>MERPQPDSMPQDLSEALKEATKEVHTQAENAEFMRNFQKGQVTRDGFKLVMASLYHIYVALEEEIERNKESPVFAPVYFPEELHRKAALEQDLAFWYGPRWQEVIPYTPAMQRYVKRLHEVGRTEPELLVAHAYTRYLGDLSGGQVLKKIAQKALDLPSSGEGLAFFTFPNIASATKFKQLYRSRMNSLEMTPAVRQRVIEEAKTAFLLNIQLFEELQELLTHDTKDQSPSRA[2x]

The heme oxygenase (HO) system comprises two active isozymes (HO-1 and HO-2) which are involved in the regioselective, oxidative cleavage of heme at the α-meso carbon. Cleavage results in the release of equimolar amounts of the gasotransmitter carbon monoxide (CO), ferrous iron (Fe2+), and biliverdin, the latter of which is reduced further by biliverdin reductase to form bilirubin. Of the two active isozymes, HO-1 is a ∼32 kDa stress protein found to be predominantly expressed in the spleen and inducible by a variety of stimuli including heat shock, heavy metals, heme and reactive oxygen species (ROS). Our laboratory has been focused on a program aimed at the design of novel, non-porphyrin based, isozyme-selective HO inhibitors based on the structure of (2S, 4S)-2-[2-(4-chlorophenyl)ethyl]-2-[(1H-imidazol-1-yl)methyl]-4-[((4-aminophenyl)thio)methyl]-1,3-dioxolane (azalanstat), which was discovered as a potent and selective inhibitor of HO. This program has resulted in the discovery of several novel, azole-based compounds, deemed QC-xx, which selectively and non-competitively inhibit HO without affecting NOS or sGC, except at high millimolar concentrations, and do not induce expression of NOS, sGC, or HO-1.

Thus, to exploit this putative interaction, we modified our strategy and QC-308 was designed to contain two phenyl groups which would occupy both hydrophobic pockets simultaneously. Initial screening of QC-308 using a CO formation assay with rat spleen microsomal fractions gave an IC50 of 0.27±0.07 µM, ∼15-fold more potent than its monophenyl analogue (IC50 = 4.0±1.8 µM,). Diffraction data were obtained to a resolution of 2.85 Å. In contrast to previous native and complex structures of hHO-1, the data were assigned to the P212121 space group with larger unit cell dimensions. The two molecules in the asymmetric unit (A and B) were virtually superimposable with a Cα RMSD of 0.391 Å (upon alignment of all atoms). In brief, the inhibitor binds to the distal side of heme in the heme-binding pocket with the imidazolyl group serving as the sixth ligand of coordination with the heme iron i.e. the anchor for the binding (Fe–imidazolyl distance = 2.1 Å). The western region of the inhibitor fits into the hydrophobic pocket which extends back towards the distal side of the heme binding pocket with the distal helix shifting outward to accommodate this region. Examination of the electrostatic surface representation of the hHO-1–QC-308 structure shows the presence of the distal hydrophobic pocket which accommodates one of the two phenyl groups. Moreover, the second phenyl moiety fits comfortably into a secondary proximal hydrophobic pocket, very similar to but larger than that observed previously. Thus, it appears that the two hydrophobic pockets serve as a “double-clamp” to stabilize the two phenyl groups in the western region of this compound and increase the stability of the complex, making for a more potent inhibitor than those previously designed.>[2x]MIKEFSDP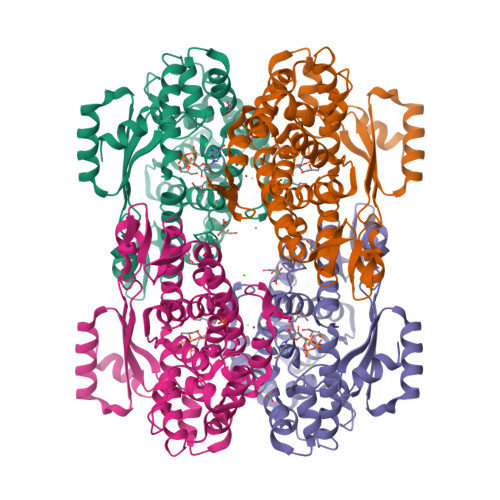LYGFVRVGEAGLRLIDSFPFQRLRYVKQLGLAYLVFPSAQHTRFEHSLGVYHITERICESLKVKEKELVKLAGLLHDLGHPPFSHTTEVLLPRERSHEDFTERVIKETEIYEILKQDYSHEDIERLVRITLGKPEDEEEKLLSEIITGEFGSDRMDYLRRDAYFCGVSYGFFDYDRLISTLRVYENKVVVDESGLRALENFLISRYFMYVQVYFHKVVRILSIHLVEFLKKLISQEDFTDINNFLRLNDAFVISELFKRKAFREDFERIFQRKHFKTLLSTENYEKFSETKERLLEKFPQEKVRFDEVEKEVYGGNIYVLSSEGLKKAHELSPLIASLKPIKLYRIYVDRQLWEKARSELKLS>[3x]MAKFFIDRPIFAWVIS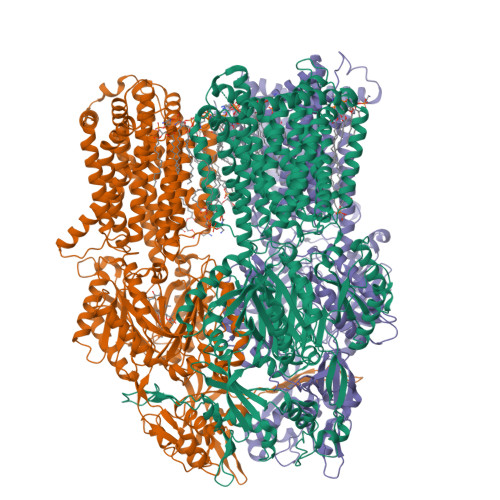IFIIAAGIFGIKSLPVSQYPSVAAPTITLHAIYPGASAQVMEGSVLSVIERNMNGVEGLDYMSTSADSSGSGSVSLTFTPDTDENLAQVEVQNKLSEVLSTLPATVQQYGVTVSKARSNFLMIVMLSSDVQSTEEMNDYAQRNVVPELQRIEGVGQVRLFGAQRAMRIWVDPKKLQNYNLSFADVGSALSAQNIQISAGSIGSLPAVRGQTVTATVTAQGQLGTAEEFGNVILRANTDGSNIYLKDVAKVGLGMEDYSSSTRLNGVNTTGMAVMLSNSGNAMATAKAVKERLAVLEKYFPQGMSWKTPYDTSKFVEISIEKVIHTLIEAMVLVFVVMYLFLQNIRYTLIPTIVVPISLLGGFAFISYMGMSINVLTMFAMILVIGIVVDDAIVVVENVERIMAGEGLPPKEATKKAMGQISGAVIGITAVLISVFVPLAMFSGAAGNIYKQFALTMASSIAFSAFLALTLTPALCATMLKTIPKGHHEEKKGFFGWFNKKFDSWTHGYEGRVAKVLRKTFRMMVVYIGLAVVGVFLFMRLPTSFLPTEDQGFVMVSVQLPAGATKERTDATLAQVTQLAKSIPEIENIITVSGFSFSGSGQNMAMGFAILKDWNERTASGSDAVAVAGKLTGMMMGTLKDGFGIAVVPPPILELGNGSGLSINLQDRNNTGHTALLAKRNELIQKMRASGLFDPSTVRAGGLEDSPQLKIDINRAAAAAQGVSFADIRTALASALSSSYVSDFPNQGRLQRVMVQADGDARMQPADILNLTVPNSSGIAVPLSSIATVSWQMGTEQSVRFNGYPAMELSGSPATGVSTGQAMEAVQKMVDELGSGYSLEWGGQSREEAKGGSQTIALYALAAVAVFLVLAALYESWSIPLAVLLVMPLGLAGAAAGVTGRNLFEGLLGSVPSFANDIYFQVGFVTVMGLSAKNAILIIEFAKDLQAQGKSAVEAALEAARLRFRPIIMTSFAFILGVVPLYIAGGASSASQRAIGTTVFWGMLIGTLLSVFLVPLFYVVVRKFFKETAHE Interleukin-6 (IL-6) is a major contributor to the progression of many chronic inflammatory diseases and a well-established target for pharmacologic intervention. Mammalian IL-6 is a secreted cytokine that exerts its biologic effects through binding to two cell surface receptors, IL-6Rα and gp130 (3–5). The co-crystal structure reveals a large binding interface characterized by extensive shape complementarity between the binding partners in which the SOMAmer engages IL-6 through two distinct domains, a stem-loop domain and a G-quartet domain. The SOMAmer·IL-6 binding interface overlaps with the contact zones between IL-6 and its two cell surface receptors, IL-6Rα and gp130, thereby providing a compelling rationale for the potent inhibitory activity of the SOMAmer against IL-6-mediated signaling.

We obtained two crystal structures (referred to as form 1 and form 2) of the human IL-6 protein bound to SOMAmer SL1025. Form 2 was solved to 2.55 Å and contained two molecules of IL-6 (chains A and C) and two molecules of SOMAmer (chains B and D) per asymmetric unit. The two structures are very similar overall and could be assigned to space group P32 (see Table 1 for data collection and refinement statistics). The form 1 complex can be superposed with both complexes from form 2 with a root-mean-square deviation (r.m.s.d.) of 0.431 Å spanning chains A (IL-6) and B (SOMAmer) over 898 atoms or chains C (IL-6) and D (SOMAmer) with an r.m.s.d. of 0.456 Å over 945 atoms. Similarly, the two SOMAmer molecules in form 2 align well, with an r.m.s.d. of 0.537 Å over 655 atoms. Both form 1 and form 2 structures lack the first 13–15 residues of the unstructured N terminus of IL-6 as well as residues in loop regions connecting the helices (form 1 amino acids 48–60; form 2 chain A amino acids 44–60, and chain C amino acids 44–59) and at the C terminus (amino acids 131–135 in form 1 and amino acids 131–140 in form 2 chain A and amino acids 131–135 in chain C). In form 2, the number of disordered residues in chain A is 18 and 21 in chain C. Additionally, nucleotides 19 and 20 of the SOMAmer have no discernible electron density in form 1 but can be resolved in form 2. Because the form 1 and form 2 structures are nearly identical, the analysis reported here was done using the more complete IL-6·SOMAmer structure in form 2, specifically chains A and B. The IL-6·SOMAmer complex composed of chains A (IL-6) and B (SOMAmer) is shown in Fig. 1A. The SOMAmer interacts with the N- and C-terminal poles of the IL-6 four-helix bundle, wrapping around the protein perpendicularly to the long axis of the helices. Each G-tetrad is coordinated by a presumed sodium ion that sits in the plane of the tetrad.

>[2x]MAPVPPGEDSKDVAAPHRQPLTSSERIDKQIRYILDGISALRKETCNKSNMCESSKEALAENNLNLPKMAEKDGCFQSGFNEETCLVKIITGLLEFEVYLEYLQNRFESSEEQARAVQMSTKVLIQFLQKKAKNLDAITTPDPTTNASLLTKLQAQNQWLQDMTTHLILRSFKEFLQSSLRALRQM> DAQPRETWGKKIDFLLSVVGFAVDLANVWRFPYLCYKNGGGAFLIPYTLFLIIAGMPLFYMELALGQYNREGAATVWKICPFFKGVGYAVILIALYVGFYYNVIIAWSLYYLFSSFTLNLPWTDCGHTWNSPNCTDPKLLNGSVLGNHTKYSKYKFTPAAEFYERGVLHLHESSGIHDIGLPQWQLLLCLMVVVIVLYFSLWKGVKTSGKVVWITATLPYFVLFVLLVHGVTLPGASNGINAYLHIDFYRLKEATVWIDAATQIF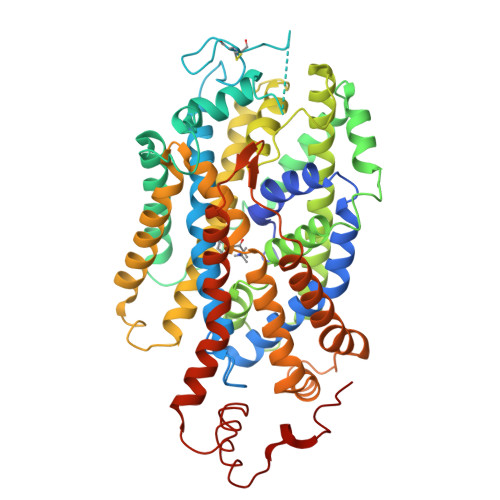FSLGAGFGVLIAFASYNKFDNNCYRDALLTSSINCITSFVSGFAIFSILGYMAHEHKVNIEDVATEGAGLVFILYPEAISTLSGSTFWAVVFFVMLLALGLDSSMGGMEAVITGLADDFQVLKRHRKLFTFGVTFSTFLLALFCITKGGIYVLTLLDTFAAGTSILFAVLMEAIGVSWFYGVDRFSNDIQQMMGFRPGLYWRLCWKFVSPAFLLFVVVVSIINFKPLTYDDYIFPPWANWVGWGIALSSMVLVPIYVIYKFLSTQGSLWERLAYGITPENEHHLVAQRDIRQFQLQHWLAI>MKKLTIGLIGNPNSGKTTLFNQLTGSRQRVGNWAGVTVERKEGQFSTTDHQVTLVDLPGTYSLTTISSQTSLDEQIACHYILSGDADLLINVVDASNLERNLYLTLQLLELGIPCIVALNMLDIAEKQNIRIEIDALSARLGCPVIPLVSTRGRGIEALKLAIDRYKANENVELVHYAQPLLNEADSLAKVMPSDIPLKQRRWLGLQMLEGDIYSRAYAGEASQHLDAALARLRNEMDDPALHIADARYQCIAAICDVVSNTLTAEPSRFTTAV[3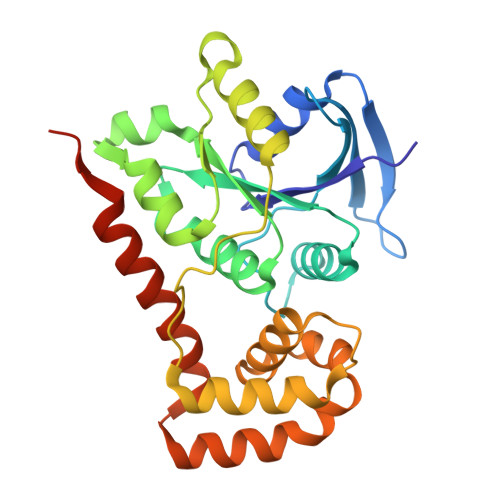x]>[8x]GSHMASMTGGQQMGRGSMNTE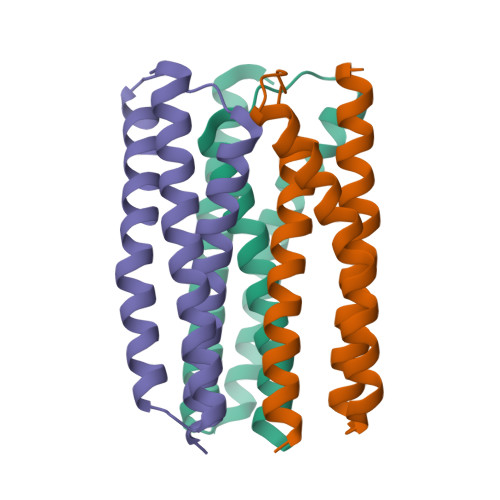ELQVAAFEIILNSGNARSIVHEAFDAMREKNYILAEQKLQEANDELLKAHQAQTDLLQEYASGTEIKIEIIMVHAQDHLMTTMTLREVAIEMLELYKKS Remarkably, this modification is regulated by only two antagonistic enzymes: the O-GlcNAc transferase (OGT), which transfers the GlcNAc moiety onto acceptor residues from the donor sugar nucleotide UDP-GlcNAc, and the O-GlcNAc hydrolase (OGA), which removes it. OGT is a multi-domain protein with a catalytic core at the C-terminus and 13 tetratricopeptide (TPR) repeats at the N-terminus, making up about half of the enzyme. Here, we exploit a novel approach to covalently trap OGT-substrate complexes to explore how OGT recognizes glycosylation substrates through its TPR domain. Here, we used a fusion approach to trap OGT-substrate complexes to investigate the role of the TPRs in recognition of glycosylation substrates.

A well-characterized OGT glycosylation substrate is the TGFβ-activated kinase 1 (TAK1) binding protein 1 (TAB1), a pseudophosphatase involved in the TGFβ-mediated inflammatory signalling pathway and found to be an essential activator of TAK1. We have recently discovered that TAB1 is dynamically O-GlcNAcylated at Ser395 in the C-terminal domain. The O-GlcNAcylation sites on the OGT substrates TAB1, collapsin response mediator 2 protein (CRMP2) and casein kinase 2 (CK2) are located in disordered regions close to the C-terminus. The structure of the OGT in complex with the TAB1 C-terminal domain combined with mutagenesis studies reveals that OGT recognizes the TAB1 substrate, and by extension a group of glycosylation substrates with similar disordered regions, through extensive essential interactions with the TPR repeats. The TAB1 C-terminus binds in an extended conformation in the TPR domain, making extensive contacts with the concave surface through regularly spaced asparagines in OGT. In this work, we have shown, using crystallography and site-directed mutagenesis, that the OGT substrate TAB1 binds the enzyme in the same way as the proteolytic substrate HCF1 and that the five asparagine residues found on the concave surface of the TPR domain (Asn321, Asn322, Asn356, Asn390 and Asn424) are important for binding. Although the similarity to the HCF1 peptide binding mode and the presence of glycosylation on Ser395 suggests we have trapped a physiologically relevant TAB1:OGT complex, we further tested this model by structure-guided site-directed mutagenesis in the context of truncated OGT (312–1031) and TAB1 (7–409) as separate proteins. Two types of OGT mutants were generated: a single-point mutant in the active site (K842M), known to be essential for catalytic activity and a quintuple mutant where the five key asparagine residues that form the bulk of interactions in the TPR domain (Asn322, Asn325, Asn356, Asn390 and Asn424) were all mutated to alanines (from here on referred to as the 5N5A mutant).

> HHHHHHVPYSSAQSTSKTSVTLSLGGGTHADSLNNLANIKREQGNIEEAVRLYRKALEVFPEFAAAHSNLASVLQQQGKLQEALMHYKEAIRISPTFADAYSNMGNTLKEMQDVQGALQCYTRAIQINPAFADAHSNLASIHKDSGNIPEAIASYRTALKLKPDFPDAYCNLAHCLQIVCDWTDYDERMKKLVSIVADQLEKNRLPSVHPHHSMLYPLSHGFRKAIAERHGNLCLDKINVLHKPPYEHPKDLKLSDGRLRVGYVSSDFGNHPTSHLMQSIPGMHNPDKFEVFCYALSPDDGTNFRVKVMAEANHFIDLSQIPCNGKAADRIHQDGIHILVNMNGYTKGARNELFALRPAPIQAMWLGYPGTSGALFMDYIITDQETSPAEVAEQYSEKLAYMPHTFFIGDHANMFPHLKKKAVIDFKSNGHIYDNRIVLNGIDLKAFLDSLPDVKIVKMKCPDGGDNADSSNTALNMPVIPMNTIAEAVIEMINRGQIQITINGFSISNGLATTQINNKAATGEEVPRTIIVTTRSQYGLPEDAIVYCNFNQLYKIDPSTLQMWANILKRVPNSVLWLLRFPAVGEPNIQQYAQNMGLPQNRIIFSPVAPKEEHVRRGQLADVCLDTPLCNGHTTGMDVLWAGTPMVTMPGETLASRVAASQLTCLGCLELIAKNRQEYEDIAVKLGTDLEYLKKVRGKVWKQRISSPLFNTKQYTMELERLYLQMWEHYAAGNKPDHMIKPVEVTESA> GSHMAKEEIIWESLSVDVGSQGNPGIVEYKGVDTKTGEVLFEREPIPIGTNNMGEFLAIVHGLRYLKERNSRKPIYSDSQTAIKWVKDKKAKSTLVRNEETALIWKLVDEAEEWLNTHT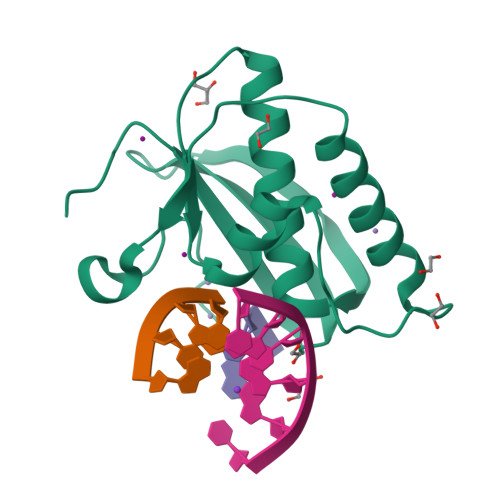YETPILKWQTDKWGAIKADYGRK> GPDEARRQIVSNALISEIAGIVDFVAEEQITVIEQGIEKEITNPLYEQSSGIPYINRTTNKDLNSTMSTNASEFINWGAGTSTRIFFTRKYCISTGTQGNYEFSKDYIPCEEPAILSNSDLKIDRIDFVATDNTVGSAIERVDFILTFDKSNANESFYFSNYVSSLEKAAEQHSISFKDIYVVERNSSGAAGWRLTT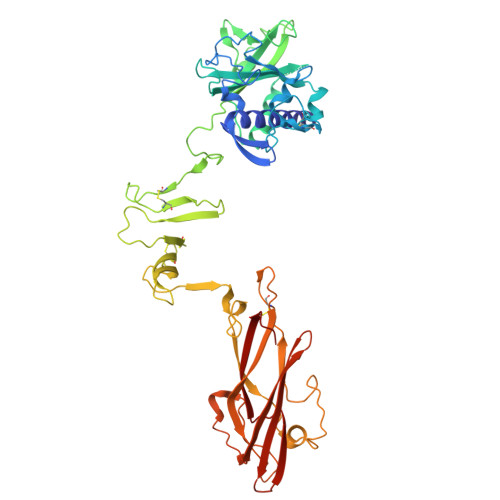ISGKPLTFSGLSKNIGSLDKTKNYGLRLSIDPNLGKFLRADGRVGADKLCWNIDNKMSGPCLAADDSGNNLVLTKGKGAKSNEPGLCWDLNTGTSKLCLTQIEGKDNNDKDASLIKLKDDNGNPATMLANILVEEKSMTDSTKKELRTIPNTIYAAFSNSNASDLVITNPGNYIGNVTSEKGRIELNVQDCPVSPDGNKLHPRLSASIASIVADTKDSNGKYQADFSSLAGNRNSGGQLGYLSGTAIQVNQSGSKWYITATMGVFDPLTNTTYVYLNPKFLSVNITTWCSTEPQT>MLFRAVLLCAALGLSQAANPCCSNPCQNRGECMSTGFDQYKCDCTRTGFYGENCTTPEFLTRIKLLLKPTPNTVHYILTHFKGVWNIVNNIPFLRSLIMKYVLTSRSYLIDSPPTYNVHYGYKSWEAFSNLSYYTRALPPVADDCPTPMGVKGNKELPDSKEVLEKVLLRREFIPDPQGSNMMFAFFAQHFTHQFFKTDHKRGPGFTRGLGHGVDLNHIYGETLDRQHKLRLFKDGKLKYQVIGGEVYPPTVKDTQVEMIYPPHIPENLQFAVGQEVFGLVPGLMMYATIWLREHNRVCDILKQEHPEWGDEQLFQTSRLILIGETIKIVIEDYVQHLSGYHFKLKFDPELLFNQQFQYQNRIASEFNTLYHWHPLLPDTFNIEDQEYSFKQFLY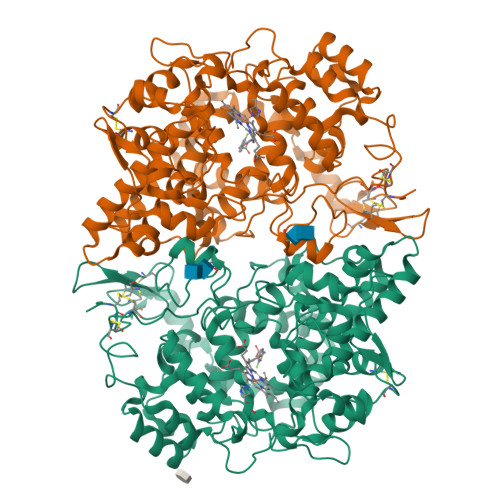NNSILLEHGLTQFVESFTRQIAGRVAGGRNVPIAVQAVAKASIDQSREMKYQSLNEYRKRFSLKPYTSFEELTGEKEMAAELKALYSDIDVMELYPALLVEKPRPDAIFGETMVELGAPFSLKGLMGNPICSPQYWKPSTFGGEVGFKIINTASIQSLICNNVKGCPFTSFNVQDPQPTKTATINASASHSRLDDINPTVLIKRRSTEL[4x]> MGHHHHHHMMKTKLPILGVLGGMGPVVTAEFLKSIYEYNPFIDKEQESPNVIVFSFPSAPDRTGSIDSGKEREFIDFIQV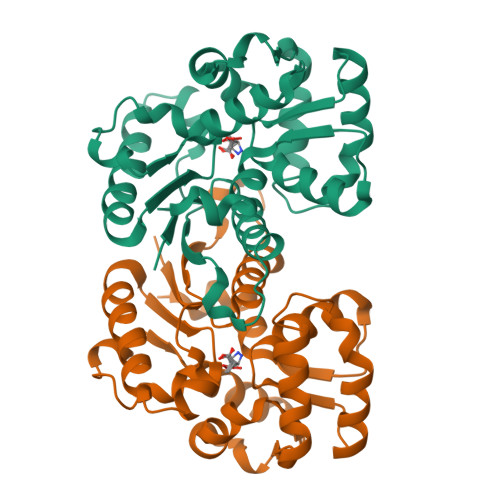NLEHLNKLADCIVIGSCTAHYALPQIPENLKDKLISLIKIADQELQEYNEPTLLLASTGTYQKKLFQEGCTTADLIISLSESDQKLIHEMIYKVLKRGHDPLSILRDIEALLEKYNTRSYISGCTEFHLLTKSLKLKGIDSIKAIDPLSTIAQNFSQLIIKQAQVDLVTDCHQPSNPKSP>GTTSQKHRDFVAEPMGEKPVGSLAGIGEVLGKKLEERGFDKAYVVLGQFLVLKKDEDLFREWLKDTAGANAKQSRDAFGALREWADAFL[2x];> GDNYADLSDTELTTLLRRYNIPHGPVVGSTRRLYEKKIFEYETQRRRLSPPSSSAASSYSFSDLNSTRGDADMYDLPKKEDALLYQSKGYNDDYYEESYFTTRTYGEPESAGPSRAVRQSVTSFPDADAFHHQVHDDDLLSSSEEECKDRERPMYGRDSAYQSITHYRPVSASRSSLDLSYYPTSSS

Barrier-to-autointegration factor (BAF), encoded by the BANF1 gene, is an abundant and ubiquitously expressed metazoan protein that has multiple functions during the cell cycle. Through its ability to cross-bridge two double-stranded DNA (dsDNA), it favours chromosome compaction, participates in post-mitotic nuclear envelope reassembly and is essential for the repair of large nuclear ruptures. Phosphorylation of BAF by the vaccinia-related kinase 1 (VRK1) is a key regulator of BAF localization and function. Here, we demonstrate that VRK1 successively phosphorylates BAF on Ser4 and Thr3.

We also verified that pBAF still interacts with the LEM domain of emerin. We observed by ITC that both BAF and pBAF bind with a Kd of about 1 μM to the purified LEM domain. We even obtained crystals of the complex between pBAF and EmN that diffracted at a resolution of 1.4 Å. Determination of the high-resolution structure of the complex confirmed that BAF and pBAF adopt similar 3D structures in the crystal. At this resolution, the two phosphorylated side-chains as well as the Lys72 side chain were unambiguously positioned, and a salt-bridge between the side chains of pThr3 and Lys72 was observed. On the emerin side, only the LEM domain is visible in the crystal, the disordered region of EmN being probably proteolyzed during crystallogenesis, as previously reported. The position of the LEM domain on pBAF is similar to that observed for the LEM domain on BAF, as illustrated in Figure 7B. Consistently, a salt-bridge is present between pThr3 and Lys72 side chains in the 3D structure of pBAF bound to the LEM domain of emerin. Determination of the high-resolution 3D structure of the complex between pBAF and the emerin LEM domain confirmed that BAF and pBAF bind similarly to this domain. At the opposite, its interface with emerin is distant from its phosphorylation sites and exhibits no chemical shift variation upon phosphorylation.>[2x]MQ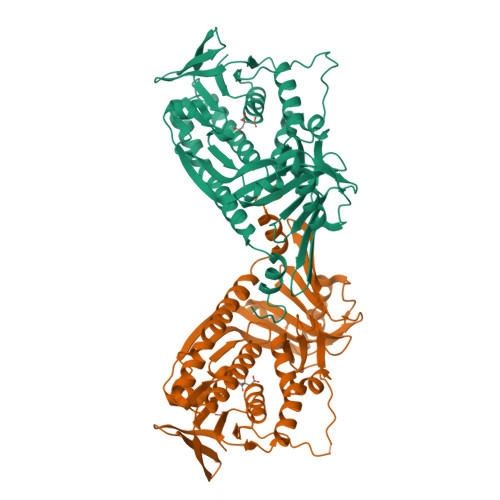QQVIIVGGGMVGLSLSLMLAKANIAVKLLEAVKYPNYDDQNVAPYHSSFDARNTALSRRSVQIYQKLGLWDALQQHATPILQVHITEQGSFGKARLVAEQEKVESFGQVIENAWLGRVLLTQVRQQPLIELIDGVQVTALTQDAEQVYIEAQRGDEILKLESKLLIAADGRDSFCRQAIGVGVDVHDYDQVAIVTTVQTSKPHEHVGFERFSALGPLALLPLPGEYRRSVVWPVKKGTEGEWLGEENDQHFLDALQKTYGDRAGKFEKTGKRFSYPLSQVLAHKQAVGRVILMGNAAHTIHPVAGQGFNLCLRDADVLLRYLVNQLSASDDIGNPDNLLAYEQARLSDQQRVIKFCDTVVRGFSNQNPLLKLIRNTGLIAFDVIPGVKPLVANYAMGLKA> GPLGSMTSKLLPGNIVYGGPVTERQAQDSRSLGQYILDKYKSFGDRTVLVDAVNGVEYSASFMHKSIVRLAYILQKLGVKQNDVVGLSSENSVNFALAMFAGLAVGATVAPLNVTYSDREVDHAINLSKPKIIFASKITIDRVAKVASKNKFVKGIIALSGTSKKFKNIYDLKELMEDEKFKTQPDFTSPAANKDEDVSLIVCSSGTTGLPKGVQLTQMNLLATLDSQIQPTVIPMEEVTLLTVIPWFHAFGCLTLITTACVGARLVYLPKFEEKLFLSAIEKYRVMMAFMVPPLMVFLAKHPIVDKYDLSSLMVLLCGAAPLSRETEDQIKERIGVPFIRQGYGLSESTLSVLVQNDEFCKPGSVGVLKVGIYAKVIDPDTGKLLGANERGELCFKGDGIMKGYIGDTKSTQTAIKDGWLHTGDIGYYDDDFEFFIVDRIKELIKYK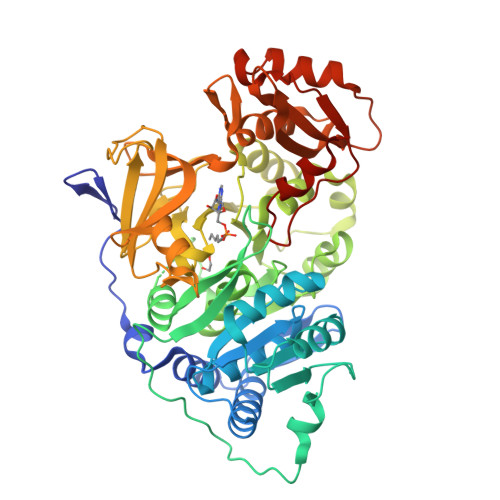GYQVPPAEIEALLLTNDKIKDAAVIGKPDEEAGELPLAFVVKQANVQLTENEVIQFVNDNASPAKRLRGGVIFVDEIPKNPSGKILRRILREMLKKQKSKL> MFRRGLVHRRYPFNKRGPRERKSWKHHVLTDPPKPIQWRDPKVWTKDLTTMKSFDAPQWDLWQSRARSEDIDEALQPFMDMPQSLKDRRYDIPWWANPFGAWYLQNILSVELLKLPSRTNAEKVAIYRNQKHSLSSKKKGEAAQDDEILANIIKERWRTLEFGDRDAGYPCTFSDYIQFLNEWFKSLDEEGMQRLREHFDRRIRPLLAVMSPVDILWLEALTQNSPHNKEQLQRRIAFQTSLGTPEFFDMSKRLRYEINEDYKVRDELGPELFALWSKAPERWPPERLSKMYGLDFTLVRKILVWHHFKACYDACVEPDWTLPKRLFALEWIRDVRARKHGLFYGKMRFAEQKITFYSDRFLFRDLVNRREASYANVWEMDDPYRFLQTEQDYEDYWGDNYDVYRRMFPEMIGKSGEPVQQYGQMPVWTGPHRQHANKSQHNWMFAEIGVNVGHEALKKLELDPTNEKRRRFVIRQPDGTLRSAKMSEMRAWYWKEEWADFRFWAPNMEWGIENTPSQEQYQEHVPDTPDADFRKQRRIQSRPVKWFYESHYTRTGNFAGFQPLRFMQRRTEREVRWPDVINAAVQIQKRKPDAYIFKAIPEI;> MFHFTVGSLKNLNSWYAKGTMRGGVPRIYYAWMRPGSFTRRRFEKMRNPFVDLETGTSLYFRDTRDSAEAVAHAADSKGLKGMDNAIDLYNEYRIVPDLYPEGFQWKHKLNTEYNQWRSNTWLTPDLIPQEHRGRFLCNFQLNIVAYDMRVVKFSPKDHRQWIYCVLYVGSGKGIAGWGRAVAPSTQEAKKEAIREAFSNIIAVDLEQEGPMYPVRVNADGVRVLLYPAKRIVANFRVADILCAFGFQHAGCRINLKATNNPKSPTHTVEGVFEAVKALRSVSEIAASRGKVPHSLIYNIYPYLEEIRRRKGMMAMHPPGKDGLLMPDRVVDNRLPDHLKKGYYDDVYWKDFFAGSREHLNEPKMGLRGDEMRQRLESAQSRPISSSTGSGRRTLEDVLKRLGKTTKDLGSIPIVNPRLDIKLPTHIKRNYSLH;> MYAHVVSWTLFLHVFFFFLSLSRTLFFFFFFFVCLFFPFLCVYLEEEMLRRLVSSHGCSNGGGTNGGRCVRPVKEEPPVFSSLVLQRRFSFKYATKLQHDEMRQPFYIHEKRHGIFSNEKNIRKSRRGLPFITPLYTRHMNLWETDTDASKNRFFRGYVFGQRELHQLLGRPHGFEANNTDGSNDISAYEMTTDQRYKGIPRPAITNLHYEPEWNYTLYRAGTHGSQLSNPRSPLTAEVLGDELMKIRDIKSFDHCKAWFDRLQYLIKLHYDAVGDIGEFKSRHTQHVHEFFVAFHDALSSFDFGDSYLFEQFHAARPSELTDLFGIFLEMEANYVHEDYCPRCSLPYSTTRYCGEGDANTPFRKHRGRWAPHQRWGREWYAVVARRAEALWYRATEDPYFGTPQHTQRQAEALLRVYVQTKQRGKAIDFMNALRGSKEFLLGSICITPEMQESYDRLLDTTPHPHLLTNGFTLESNAAKYTGEVQKVPFSPLQFRIDMEMNKYRRQQKEEGAVRVPPAMWRIDTSAIVPYKVDPKTKRVINWREVKEGIEKSFLSTGLPKEAYTGSEWREMLHLKSIIAGRAAKAAELERRLHTDKVKLLEVSSKSKIASETNTSTGSSNSSSIIFPDKDGYHVFDTSVASLRPFGVSQSGAVFQSVTHTYPSPHAVLYNDPVHGKQFILDTTNESCHLFGGFEHGDRLLIRARKIDKNDNNPNSVLAVKGNEFEVIVVGVNKEGSDSEWQLCAMHVDPALQREYGLVFLGTDCVDIHERWASVRYAAAAPHVKGRVTLLEERRTAREESLGQIVGVRDGVLFVQWRLLRGGGSEMDRSVAEPIGTVEQVRNAYQITEQGVEELMHPPSWRTPFRNDFAEERLEELRQAPFKRENWVSLIQGRYTPKLKRFGYTQHTTMDDFETKEYKDRLLSKQFFHNPQAFEVIPDRRDRAVTFGGKWEYQRTHGLPTVDRNELENGWSEVEAVTDAEMHVIEQALRDISGRRPGNFIKSPTKKNTLQLNESWWEPLEFGWEQHNKEQKALVDPTEQRLIDSASLPFGGKIPPFGTTIGIGERIREIAEDYAKGFGLGPHGHSPSHDTCQYNTLNAEEDRVRELGYKDALVRLFDEKMADKDVHQWAVEQCADGEADVRQLLLSLHEWRERGRPPSLMLLQVLSKYLEQEIAAFNEGVPSSVPKLSLQTVDGTLSPSGNSGERSGTIWADVEPTAYALQYASQANHSSLDEPFILQLLKSAQLGGRNAQFTDPFYNAYLENSVVSEFQLGLAALAGKGVSPSLLAQKISQLHRGSVRLSGNVIPFVKSRELAHLLERMGLSSENIAVVTRGLANCPEQESVGDDFAVPVSVILSWGGPGSGSSTNAADRKGNATQSRNELQRKGSAALSSAIRQLGQKRSSSKNWQNEDKMMVHVIEELALRDDGLVMDIQYIVRENRRNPVLRHEFFAALLPVFAGKHEKVAQLYDEYCEGKYVPNITLAIEAFIAFLCNVTKHADVYPGSSYFDVDTTNGPNAGQYISLKLLDPLDGPFIFDNIKAEHIETVERFKQHGIQVGPVRAPATGFIAANSKSLSYFTRRPEEVVYVSTDADQGLRRSLERSAHYKTIAASPAMQFLLHTQNGAGLVATFNRFFYRTMPMLSFYQRILKHYSDNVQPLRQKAQNSVRGLARVLENERSAAMEEFRRNSERYWRNVLEGRSVEQAMGGSGGSGGGGGGTTPPVSSSPSQSSQEAMAADVARAIGSGRTGDQKGGAARQQQQQQQRTAGDDGGVRTTFASRKGGSRSMTDLLSKLNKPKGSNTSGTAKGPTKRGNPKSHTDGGRGAKP;> MIRRRLCFVSRPTKAASISVTLFSVQRQKGGLHTFIRDARSSSFTTPRQASHAEGEHTSSSLNSTDWATQMQRELFGETDPLGGQAHKDYYRDPARGYSPQYAPRNFAEGGAISYHHAQSPMEYAEATHRRSWLDHDVARMEAAFQEQRALLRGMESATERDELARRYAAEHHVADIVVENQSLLPSTQVHHSTSTSGSALRQQAVVDRFQIADQQSPLATSDGMGREELAHTYRMRSETVHNDWIEENLRIVHGLREKEKYDFTVLQRATRIPFQGYDMDRFLAQQKGTPYGAQSLPPNTASSTMEEAQRTLRDPTATVPSFEAISQKAFARNTVRDHPTTGEELTQEVVDTIRTSREASEWQREQERAQRFGLGRQGALVQDGGPDKRTLKKHVNDERIMDAMFFRSDAYRKTQTDEHWNPYMRQDTTHGVAHLLNNKFDIARREDRLSKGEQDLTERSVMHFGVPIQQTIDEFVFRHRNARGERPLDYFKPFPGFRDFRLNRMYRDVEGFSLMKQRPEFLEWELFTRYRAHHQQRRRIALLHGLEPVANETAQERDARREKLDEICERTPFDERELHTNDDEMQVSGETLRSWFGVYMLPSPTVVEAVVGASASVNLHLFPLADEMGTADTRENVLSSRYFNRLLLMEGFQNRISRAFMGNVSGKAPEPVVQYMQPPEVLRHFTAEERAMYEQYVKEQTSKQLGEWATAMRRRRWIPDRQQYGHVVAQGYGVSVVDLEHADTAAVLTVSAKAFERELAAAKGNTSHIIMVEGQAYKLRPDSERFVVPLSVRLESGEVLDMTDEAFGRYELELLPRNVNHALNYGIGDYAYNRGNYIETQDVIWEEQTASGEEGWSPATHADGLRAGLPVRARRHVGMNANGSRIVSSPQRAVIVAYDRQPFFNPEPRLVRVAFQSDGSVEEVPLANIMIWQRRYHGPERTVGDESRRFSPASLRRYIDVSDPFNEKKSKGEHFLDKYEAARTSEVAAGKYRTTKQITEIDQWTRFDVSRADNFRPLSISHRRDYIRLGYMHRYTPWEWIAVQEADQPLIAEQIRQDNIGTSYFFSLNRYWRYKARPHGYIRHFDNEVRDLFQFVDGVTPWKQAQKIRTYWEVRAHHPMPQFNRPEVAMHRNTVGLLPAHMWETDKKTGKVKAVKDSVRDYQTKTPLPKWVQL;> MMRARRVVVALSPLAQLCVHVQWRLYTPIWQPDPAVDHVAPLRESDENRTLWASSAPIANVSDAIAAWIRFGNDPVLHTALPVIHAGQNERTRTDGSSASLSLSSLPSPSSTSPFATVEDYMGTNMVFGSPEHVKDSAAVWASYFERRYLSQLRHSRRTAANHVGLVNAPDVFTDEADRPETKWSQDTRFRERAYMAEKFLKEKVANLQQLEQALKQAKPAEYIAFHDALQQQTLTLIPLPSPSVWHYGGARRTQWAERFLPLSHEAQQFFTTVLAEDLKRAGDAPEKVLQKVAAVFAEVGKILLQRHRRCLGGREWSALAPHEKDEFCMKEVERWKQQVEVGEFDPPLDGDDDPTSTEWQSEHDAIMQLMTATIDGLSFSALEFWTHTIRCEEMETEHIHTEKRVRAISAAARRAMYDTTSYEAVLQGIVDAVAKGQLDMKAAGFKPHMNDIWCQLNYAKFGASTVTQHTTTARRQLNYFHAGLLKEVAATAALYYATKPLSSSLDYASPYKFRRSLVGLFSTYGVEMVYAVQRPLLFSAANLAKAEDLIRGVVKNVARPFGERRRAKLKQLRANHRRLATPVQGVVVSAVVSDLLESGADVSEAKKAEKMQESVTFWPLGARRVVSYDWPTPHFDALKRRVAAAGSAVTAQSTKEIQEIKRNAFVEVSLWRRVTAEETKQRRDAVEEETRRVADVVRTIPPLAQVQQYATSLYQRIEDAAPFPAATDNNAKSEQEDDESSWEFVVMLDDRVVLNANQAAELYLPYTDASGVPIPQGECRVRVRGFDVDVNPTLNPAFCSEAFSTPFQVFDAIPQLVQQFFGTAKPSVAEVSDIPSSKFIQFCAFLREAGLDVPVQCEFEAGQVLNAEGDVFMEYFLNLLRSDRFHRSCAQAGLTEMQRVIESSCRAHWEVHHPGANEAEWAEARRRVLDRAMEKEREWWFPNEMLDVTNMSPGSNHGLRLPMYPATVRYGRELCTLLAAEGQFDNNSGLSATCAVNGTGAAESITFSTGDHISSTFSMEEALAVAKGALRNAHDRQNTLAAFRLGPLSKHSQVLLFCGINATEFGGKYARTYTYAFEKAKKELAETFVSGRVVPGVDEDELLRVSDKEGVDRFASSTHPEQRKTQFVPRVGPGGAPIEDPTADQKTQWGR;> MFLRTHVERHRSGKARAFVFRDPTLKMMRAGSGYQQLRRMGMPIQVSKGWRKVDHFHANNQYQHAWPLLSHDDLGNSDQSNNTRNIMYSMYLPKRNKGTAPWFRGADTYSVKYCEQGRYEYQRYLMINRFPSEYRKHFMNFLSNIRSSSGPATIPQEALHWLLRMIVDNFNPQHVHYIAAMKTLQNAGELDMARDVWKIMERQQTWPCTSTICAYLDVCVEAGEKTWAMEAWNRYCTELKFLQPGEVDPKPVSRVPFSLTREELLYLPKWKKHFDHDPNLDVVDLNRFNRTREVYLRMAQVMLAGGERDSFQHFYTKLEEAMLSTPTPVPEPPNPHLVRRPQWSPYEHCKSVHHSPWRVGNNGRAMALGPSLTTEDEMQSRFFSNDQFLVHMLKEILRIVLQEHRRRHPEACSRGEGEAFFDQVVDARETLNFCNELIERLFAVLGQKMHGLNTSSLLSVILELYRVMGKETGMALLRRANQFLERKAALEDGAKESLTAPNYLQVLMGFADESAYVYDSKRKGLCRYRSGFDPRTTMQQLAATVQEIAGNPHVTWAADMHLQVVCTMVGCGTMKANDYFVRNVLRQFCWDSRFLEALYMEYRRHDDVDMWAELTKRALVWTARYNVNASERLKRLIEDDYDTIQVHTRTFRELAVFQFRDVEEKRHSRDVVNELPNPWTDYVSHALPFPDRDAGYPDEYGDIGQWRAPGGPGSPVKGPGYYAPPMEGEHQRGYTAEWRDLKNPMRPPEFPTPWERKYKQYARGQHPSYDMVYAGPMPEIFPNRYDFRKPTRWDFHDIEKQGKYKTSGPY;> MSVTGVFSKGRGIGHAAVTSILRYIPRARVPWQPSRFGRENLSASDLAVLWSRGRYRDGPGNYNSGYHTEKTHVLEDNTVTMIPKHELEKYMPDISIGPKALVTPVSLMSARNGHRVTHDLLHSYDPHIGRLDKPAVVDHDNITVEDPNRVGLNAATLDCRGRIYRWLRRGPFFQEDHYFRRSLRLNRDGTVPTAAHEAPLMRKIVRLAQRGHLKAACEEYRRVTTVPPVEVYRALTACCIPGGLIADAVAIFEDGNSKLFYVARDGEVLHNVMRCAIKAKNRVRVMWVYNVMRGRYYENVIVRAEIDPIWRYRIALLALEYFLDHNCAEEAGTVYSYLVEEDLLQCDVHLRVGLHMREALSKGKSVGLSDEVLRATSLVTDVATVAPEVARELYQRHVEALRENEKSNDCDMNTKNDGATGCAWSAHGLLTALDFTQKDDALPWMQQNFGDVDVASVLRWARFYHSKDLMAKDRPRYLARAVAWIELLSKRSHMMEEAPLTYMRKSKPLSLNTNSNLRVAWQTPVARPDGPPRLLAREEGYTFHHNEHSRFVTETYRHPGETLQSRFLAMQPIHTEVSAKEDFQEIYAQQQEQRALPSGVVSPTARILHHSVTSEIHGGGGGQHHRSMSRAESSTGGAVKKEKLNLVSPHVAAEKRGGSGTGNIGGTAAGGGVTPEF;> MLRRAPCLLATNIPRSAWDPAHFNTNWSDSYSTEIAARRHWPAKKWSIGLEPRTPRDWLQFSYRNLAYAYNGALRACQSFPEMLVCYKEMKQRGVKVDVDTMNVLLTRAARYERIQVDDVFLLFDELTALGARPDIAAVETLHTVLDHSAAMPYEWREARRRQLVELYNCLAMEEIERLAPHRVDRLLKEQIKRYRDNLRALKASLSPSVYRRYLHTMHSASMLLEEVHNFLWELVESDHPAMEIPALQLRIPFVGSVMRRPETDTNEKLVKYTDFEDTDVCSVFLAAAERAVDADLHDTRAVSERRIFLSLLTMISYSGVLYTSDLMAQLMEMVKYSTHASSRDSDAQRLLRYAVRGSSAAQDDLYRSLWLKVEMVADSRVLGRYIGAREPWSPIRVCFDERGLFKSYPPLVHASAKKTSAIEADATSGSGSTTMEEEQRQQSERQRMSTEITSHTSKGGEEMVEGVRGAVVAETSEASGVKDVALQEASHGEQRTVEALDLRWGDIHRLIERTRALTSPPTERHPQQEKMEIFTGIAVYLRTIATGRRYCSGEEEAGGESPAESRERALFAVGYELDVWARLFELVQEVRHDMEKFITDNAAHHVEPEFECWEALLITLRCILDFCVVRTQEKGKEERAAVEELFEKTMKLRNELVEESRTRFGGRMRILWLQEA;> MLSQNVAKTTVPSYYMIRTNLPQRKPQNQWEGVYYFGGITKRQRHLILLQRKREREARMRAFSASCSNLLRLLEGDTQEQQQAKTQTIQLSSPHGPFDLAIRLAQHGLYQQASRIVDELHQQRALRMSHYGLLIDALSAPCLGQRILYGSAQCDPALTYKLLGDENGEERAQEAHRWFDMAFALLTTECRMSGSEHRLPQATAAATHLVNALMRALLTCGYTHVSAVPDAVYDRMGLMGISPTISTYELVMLALSLQGNMKEAESVFSFLRRHHNEHVTIGSFNALLLGHRECRQFDRCDAIWQELVDRRWPRASTLTAELYLRSIVDHSYTPTSGPLQRFGNINVVEKKKIPLVLAQMDDLGIPRAHLSRPLMDEVEDALRKFHIYKSRYYEWGRAVKQFNFIEFRRRNGWMYDLHLMKNTTKQVGPLRDFNQPDATQAPVATVEIPAFFNERPAWEQPPLEETLYVTESRERYDDVRSGDIYEDRTRSLHDRSPTWMNEVPETRYDHLYGVNHPDIAKIGIRRHLNAEYVNRKEVVERDAALMKKNLSTGRRLRRKVESSRTHRNAGSMSGAAPASASR;> MRSIRGVCCFSSLYTTQFRVHATYDVAPLSHKELFSIYQNWDKTRDELDLLEEVEERISKWKLNKWEMRIPPLLTAREKELMRQQQELLKSIFFDWGKCRDALNKDLELISSITGLPKGTVREKNRAWLQEEAAKLRWVGEVSKATRLRDAFLRLEVYGSRDHRLLERLCCIYGLGLQGSFESAFSNYIVEDPITKKIYVDEKNSFRDLLAYIIHTYPQIDIIYDFLGFNFIGGYRSSLRRYLECMVSRSTEGEKIPGRLVFGRGKPAEILFDFGNSNESLVSGECTQGFPDFVFVKGSDMTLIIIASENSWLRNRQLPHRKQMEGIARRASFVLGIPFSEVRVRNLLLPPTYLDKDSIVRINEAVLGLSKEEQRNLAPWLEMYQKELDSKDVDFCSLMKSTNEEEWLTL;> MLRRTSWRAVGYTPVNPDTSPMLAYSQYHWHYNLPQGMERPHGVNRTMTAPYQSAHSLVNKYRGVWIELDMHPAFRVALEPQLRKLPQGRTIPKTSVDEVISDYINTAHLIQDEMTRDLWLAKVLQHCAFQRSNEGMALWEKYCHSRFIADGATATPPLPLVKAILFYCSKIDYQGWSSIFQKCLKNDWNYTPLFDTAQWNFLLKSVGRMGDEKGVRLILEEMLDVQADLDRVEARSIVIALNAVTDNDIYEYIKKYLFNFGERKVKFLRIIYSDLRGHGAGKLRIPLKENDKMFYHVCWHSSIRAPRQFSPRQLYFDYTPSTLGASVHNPNAKIDDIVKDKIEKWKTEGLLPEDYVHEDRVYDRGTAFKNVARQEKWKKMPRIVKSKKMGYTGDP;> MSFRYTNGLVGALKHRMMLESSHRELVRRRFTGHCRGVEVVCSGYGTVLAVRLVDKTVWEPFYRKGHPSPSGADMDSAPPSSHAEGTPVGGQSAAPLDFERIAESIKAALWDATRKIRSAKEAALNRSLSHNQQLRAQAHLEHWYDEDANTLQPLAFEALKHEAATPWMQFVQFGKYKHAAAVMHSESGGKTSEAFTGETKRAGADNEEGPCVTALDEKDVDPTSIPIGSVHPLFLPALIQFESRVDNSLNDDAIRQEQRREMSRDEQLFWERVELIRKGQVATIKGGHKRDYADEAAVASDNAVDKVQLRFTQ;> MMRCCCVLQDKSMFAAKRRVIVPIHPTPNYPAHFIKASFTTDPLKEKQKARFSSGGEAMREVQMIPKNLEGERSRRELMSRGDTEFEALVEFIQGASYDQLISGRRFKKVYDKLSENDDTFVWLCHTAMSVLNPGDVRSRLVYNHLRTLAEAVANGEMTLRTAFRFYESAVRSPAYREIAKRQMEGGAATRLAGISAAADVMRRMGLTRRPMASYFELYQRIVERSEAMTPWGFPPLFQFEERLSLEPRLKFFSRASQQALERRRRGHIMSAYTTLQGRRIFWIPPTWNRAGRFLGPHVTLYPGMTPD;> MEVYRRITERVRGALWAHHGRLMSERQFHRILAYVYNNKYEHQIRFDRMEVVGRAWEGRVEVVTTPAGYLKRVRVNPCLEELSSYRQQQLILAAYADACAQGRRLMEKAEINIYKQFLKDLKPIVMGIRDNPEFYTVPEDSVETVGGTLHMGQGPTPTTYRTIPAAKAHIPVDEIRARQEWEKKWLNSPQGQSWALTLRGKRYFALHGPQYRPRGAPGAKKVTMPLDLPAPYTSMDERRLLKKNWMAYLDNKHVAEVMWTRAKIADREKLQRRLQETGQAWHRPINKEAVSRW;> MLRSTRPWRFRMKGGEMFVEYKIMSRDHRRSIRVEDAIVDPSVARTVVPLSWLEQLRSPSLRLHTGYHMEEAVYVPPAYAAVDEKEGRRLSEKSTMTPNAILAGPVVLSITGQSVPVVLNPYFVPDDTWGIRRNRDEWDLRLGMDAIEQCTLFSELRPGGLLYNKLPSSQNVTRHEPVRATLQRYGMKCGLAESPLVPRPWTRMRYMFIDELQRGPKLTEFVGHNPRNGTQWRFSQHSKYFRIGVWRETIRRNDMNEGLHGHSSWQKSPQQAVPEVRLMAPYP;> MRRFCFPVATFAQAALRHRGIRWNTTMADNESHTGAKSSASSSTPSEANEISAMERASEARREIHDLWMSTEKMLDLENRVRSVASLIEKYKLDPSTPRENDVSRGLGDAFDRLLLLCVPLGKDSSKGTDDLERLMNLAGRNGREISVRTIQHLFARTDSFSEALAVFYAMRRCHVAMNMEAYYAMLYSLQRLEEEGWAQRFREECEEKGGVSEQAMDFVVKGINNALLPENKPWLGRVMFGDRDAPAQRREARDYDELSAMWTERYRDGSAFPTSP;> MLHGSLPSLASLRYRRPYWMLFLKDVDNWKIYTVIQQPDHQRTEMLYQAWLGGLDRPYTRPKCMANQPLWLSKKRHILRKDRLDGPETPLEKYVLEWHKRFHSFQGTERPTVDDLHTALDLVERPLDLSYAFQLLNQCRNVNNIRFAKDTFLVFLEACLRVDRKDCALYATENAEALGFWHIEEDYRRYLRGEQSWYRLSPLDNMYYPLEENVKLNAGRSPPSSAAVAEGDAEGTAETTGFEAAAGAAAWSDDEGSMKAGSSRESMTVDDEIARLEAELAALEEEGTDGDNDVKGPKGH;> MLRRTFAVVQKGERGLYFPINHRIVDRRIASGVTVEEADVQSRYRRELRTSFATGETRQTIPPAWSACERPTHFLSLRLPVRNVLRTRVNEMHNQILFSHQQHAPLLVPLEKLHITLGVMAISEREETERLASIYDCVSEVFSVIHPLQLRFRGLGTFGFGRVLFIRVVPEADFGILETAVSKIRRRVGGELKVDMKGNPHDSYVPHVTIAKIRSKQQTQFGSKIPISMWVEYQHHDFGDVTFSQVDICSMRGSKDGYYHTEGSVHLL;> MFGRSALCLAKRFRYNTKYPSLVSYNKLPWEILNHETPEFHMHVAPHYEQIMTLAASTHVPHIVGKKHLEMPPEHRLRLLPGMFYMLDGDSIPEGFTANRVLDPTALQYYGRLESLVAPVQAVRMLISDDLRIVCNSVTLQGPLQLPVASYASLASLEVVTNKASASFTLFHFVRPNRPPSELQLEKYYIHAPRAMALAEFNSTSNTSWEPKLQAPKRSKRVTPLPAYRPPQSYLMGLAERLAVVPGSSFGRRSLMWGHWF;> MMDRTRLFLAAEFKQKSRWSSVWPNMHYGAMYLSYSIGRKLPMKGVNWVTRESNRLTNFSNRYQAVINDIDVKKTEEELGITLQDIRWNDHRRIYWKCSFCGSSYRKSVSVRTKFHAGCNFCKGRYPSEVLREQHQSLSLAASAPELIKQLKETDKKDNLGSLALTSKFRAEWKCQSCGGSYRASVRSRTGMVENGQCPLHPNIVDWSAYCPSCSWRPNMEAIAEEVQRTGQFLGLEAESRKIASAPPARIPRRKKLVS;> MLVSCIRRQADRRTRHHMMLDGQINPREWMNWHPKEYQPWYFDRHKFLYERQQYAHFHHLLCHQVFLKDMLHLVQHPEPYTHIVDCRTSPLKMHRWVPHSWWLPRDEVEYALQLTPDEFADMYGFHKPRKSDDVILVSHNGLYSEQAGWEWKKQFYQHVYNYRGGTNELFGEQYNDVALKDSLPPWKGPFPQSGIFVDKWSKRKVLTRTGPFDRQYEMQDFALPDLELERPRHPEEGPRQNMPYGLQ;> MFRISPSLAWRRTAAFYLRAGKLGQYEREAFEARRRLEESKNYPGPIRSATPGDTRFYAGSLESILQDNDRHYWRAVIDDPQVQYVIPLRIRFKLFTWVTTGWEQRLHIVQTMAPRDITIARLIELVTIENQSPYLCSSTFTLAVDGKELDPDKSLSDYGITEHSRIDAIEKLDHLLHKDSERPLDWTVDEMTTECLKRSPYKEMGMQPQPNLAPRYEARPKGYFGRNNYSGMKQES;> MQRAGCGIVRPGRGCHTTPLYCSLATISTGVFDHLPFQHRRQHAFNTLPLHDANHFGGRTAYLREIGPVNIKKSGRRFKKDLRTVQFNVDIWCAQQTLRKRWKQRDWEVIEVPFRLAPAEQQRVIPEMYTDVPPMTDPERHDFSNIRNKVYDREELQGVLFGASGPLPYPPLQRIDRQAMTLDKFL;> MRRTIAALTATPERFSILGTTHPKPKRTGFGRNNKMRSKPSDNVAWYDKGPVEWLPRPVRLTYDHLDQLRDWMMRETLDGKTEEFNRIRDMHREWSQHPLMPVLGDVEPKFPLNLFKQNHRAKRRFLVRWHKANTPANWLWMPRGPTVVTPLHHTNPSQYPESWRQMVRKKK;> MYCYYLHTSPASNENDVCHSASAKSNFIFPSFSSLVGFIVFFLWKRQMPLFHRLFVSGADLRGCHTALSSTFTQRRYWAKPKKRPKVGQGFHEKAQKWRDEFLLDRHRILADSLRAYVEFSASKRTEPWDTRFRPFDRVEKDGVYVLMRHLMEDKFQLCNYHHRPVKRLFCNVGLLGPQVTTKARWKPYRYATNPANTSKAERIFQKDKTLYTHGHND;> MFGTTRVWRNTFLTKSVATPPISVIRTGPKWWADPERMVRQKLMYFTLGVDQLPLRRTAVIQKDLHRFHMCKPPPRIGDTTGYKRSRAAQLTTWYRRIQYQEYHLQHLFTRHVWGLVRAYPGNTTKIQGKADDGYVGYDSVPYHRYNRTPLPFPAREIYGRRE;> MVFYAFVLVMKPRQRRFTSQALREIAVAIYNNGGLIRKLSNEGVMRPYSRFRDADNTPLTYARYVTLQVDMGEEQMRKVEKIMKEHQDVFITLNLNNLERPVGIRRGRKDLQSAYFPLDTFTRLEEEINWPPQTSADIYKQLEMNWKEFSRTRWSNFLRN;> MITELRTKGATRTPAIRYSYPAPPPSKNAAPQQPRGTPRPRTAKTNVRKPKRSDARRRARAGSGFGVVSPVRARRRRVVGPPFADFFGALFPATRGIAFLSDLPTHIFSSFLLSFLAGRGVAMLRMCRRLAMKYADLELTTRGEFPHGMKEPGFVKKLDQNIPWYFSTYRSMYHWPITGDNWSDLNEAEKHHDLHMFYTLAWWKLGEGIFDANDEDN;> MRGCGVLCAGHKRAAVIATTTCSLGPPTLSPSLTLRPVACAATPVTIPIFPPPMRGSFIDRNPVWASFNEKHTAKSFRHRIVSSADVSLRPPQFYLSNEKVSAGEAAVVQKRAEATDSYGEQLDEISARWAAKFYGRVTFGPRNYPYPSSRWLARRFKMKKHRIIKRFRFRRYKLAAVANLPFAKMIRVGLLPELKSSKTKKGDDVEADLSGRLVSAVRSSGGKKKGNRGRPKSKYQI;> MKKMVFCKMCRPLLVFCATSCWRRSARLPLPFFFSPLNLQVAPFTSWNLQARYFSTTAGGGREGTNSSEDDYVFDPTLSVQKDAAIHVAKKSLDAIVRDLLPENAPDAATQKVRAYLQQHPMDTLITQPTVHITHVEDPESGRETKMSLSPCDLSEALEQAQEREMNLVQMGTRGDVAYCRIRREIPRILGLVGPELEALREEEKQEGSSHRGGSDQAGGKIRELVDHSFRDVVDAHFVGWKSKKIVEDIKKRHPVKITIKEFQSPEAAIGKIREMCQAMQRYAEEKLIYHHFTSIVANDREVSVSFVPSLPSEKGNSWKHIKYPGEKEWAHANKRMEEACRKSGRYGTYVKNNMLKPRSLGQTFFRVDKYGRKID;> MTKKGATKILFIYKLSKLNVYNNESYKIKLLFNHLYCIDNYNSIYFNLNGILIWLNVLHINIILIKYAFLILLNNLEYLIIFKYNIISIK;> MWFLYGCCLRFVLFVLCYYMSPRLPSSGNRRVLYAVFYLYIFVWCVRCFFCGIFILSFALFIIEGGGFIDLPGIKYYTRICY;> MLRRTIVPLAKVYGAAPPNGTGQMQPARHRLLHGKRERQGSLFAIANDVKYDEKRLRQQLNAMLEEERLPPRTRLERNKANGGEALPQRRLVDLPGVERRRDLPADPITRLFFQHKGDHALYYGTYDNPSLQDEDRIQIEKREPRYWTYNVFTPVYDFCHRIREATEQRKRFVIVPSTVETRGCARVMLGHGLVAGFRDFHNDRAFAVELKYFQGDSTINVIEPCAYDGKTEFEWSPKMMRRLMNTHGIHNRLVVYICRTADNRVIDHIQAVKENVGGRGLIMVH;> MYQLLSPRTARHARLFRLANNLASSPSGTAGVPKTDGERLLWVNSHVKRNKDIEMSIEEESLRERQLPLKLGENAFTSSAQATHGSLFHFREYPMYPGEYVPAGHNTLSSLRHELRLELTAQSLKEAWMRISGGIYFQSADDYYASVDGLDAEQLGEVLAALFPYLSTYEAQALVQCTLDSISKPMNTASRQLSRTITAEAVGLDNAPGHYTNFLDWMGRLTETRGFKTEHALFQFSRRKFNRDDVRVMFENYKLMSRATLIADSADSYSHFYTVLKDFARKVAGEDSRHQIGVRIDEPEVDAETGIAVGRGCADGEKYQFTALLRENRDHNGAITIMGKPMALVLDNKAWLMEMLLMPFDEANLDYRDFDVHIVLEGHAMPSIANEIAAFALRMSIANALVKLLPLTRIPLKKSGLLSVDRRRERGQFPGYLDGKKVKRKFAKR;> MRRGIVNHYYWSRYRMPTQMPKFDGPAPIAAPQNMNSTKTNEFIDPIDDKFPLSIRGPLVRPDVPEDQYVDSWYVCTSMTHHLGDYRPWSASAPPNAYRFRPYNEFDAKGREYVEYMRQFARYDPRKSQGKGQKGFPFRDAYLTKMNEANRTTPPPTLETIMDRAVREKHQHARVLSPMQVQRDVGRSETPLPCAGNIPVDRSQFPFCWKTEDWYEYEVAKVRNKRFVFENTEEDGIHGSEVTYKIVLEGFWDHHVMKLAEDVCMFLRDVGRQVTEEKLVAVRRVMEGLTGGAFDPELIDFFNAARAGPFGRPDEYDAEEVANFVRADLKRLEEQCLNVINRCNVPVPGATNIYDPQVSWPYVEKLEPWVRMAEFWTSSSDTSFTELEMSTAHYEFRKYFRVIICKLPFQSTEFEKRMYDIRHWLHRQTTCEFHTIYRKNVIHDGSVFPTEHDPATPTTHDHHRMFSFALDWQSAPVNRLSVARVLEGDDWERVAQRLGCSVDDLKEANPAIEELEAGAVLNVPGGASRRLTSFGAAPRVLPLQNPNNGKRIRTWEDAATVLDCTVEELQQANGHAALTYKQTGENGEGEFGPSVTELNVPLSCWVSTAETEFSPVELVFAGDTFATIAQRLRCSEEALKKANDGQSDLSHARFVRVPAEAKAPRRLLEPQLRSQAATDVLMTRTIAEEAAYGIKNIPDLPSNASKFPHEYHTPTSRFPTTPKEKESESDWMAYTARYLDKQFTHPTEPTPIYNVNKLWPMQQVPGKIDQTPFEEDQTWLLNPIPVQQLEQHHPEKDLQDLPFVNHEQFPRSLEWTAP;> MRQSLVLLRRGKPRPRAGMFPDKYRRVPALLKPQQGGQQFFNQFLIRFTNDRLMRRDVEDGEDKKESKIAAQLPQMDWEHMSARSSSDAIREEMHRLVEGDAVQHQRVFNERIWYEEEERRRLQTGADAAAPTEDAGGAKEHDIPPRVLGNDYFQSRFGYSLVKQSEMPQGVTDYNQLDMWGEMPKYTRDMVFLYLISRRRNTYAVAYTYEGKRILSTYTAGNRGLKGGDRGFRSDGSTDNGHQVTSMYLNDLLPKVRELRANEGRPIGRGEKIELVVRVMGFYNGRQGAVRAVQDRANEFHVRYFEDITPFPLNGPKMPRGVFK;> MLRITSACRGGYMMYHRKSMGTMKYSKWKGAHGGVSHFYGRTPMVEEVKRNEPITLIDRRIMHYVHRSRLRHFQLFRSYQQKSNATECKLREGEMLRRRWHRKLQKSFIAFMQFKTMKVLEDQAKLVNTYGQAAVNAALGDSWDAVSDKEKDRKYVTIRRQVKALPVVSVVPKHVATMKQIHNDRFNYRWRVN;> MLRLSVGFLMRHIGQDVPKRHTHFVLESRLMYEKSFRDSWLHSVCRAVSQIDEPLSKTISGTRQKMLQRKVTCFQYNQYGLFKVPYYRLANVDRYHAVQGVPGTREWVPYANVSYWTMNKMVRSGNLLVHRVHYTGWGTDPHLKKGGWEHRWNKVMQRNALQYSRI;> MFGRTAFLLRKYRQKSKAPDLKTSFSKTRNFKKAEKIAIETVDGEVVKGRGKLRRRSHSALKKAIGEMEHPSIWLWYPWRMNPEPPTPGMPQRRALKNLHGAVFTDLTPVQKKRQEQMLYGINIPETRQMKFEQEHPLLASALRQLDGQPKGFPFWYKKYPTRRHAYGNRFSIPDEMLEGYGEEMKKALSKEMMSIQEKQFAQEAMYMERYAEHDFDTTSPAVLAVKRALKCRVLRNHLLTNPHNNIIKAVLANTEKKLSHALRKLRKVDFKKYWEIIRDHDVQDVLQPSNLVTYRQGAYWKYDWNAGLAISTNLADVLDPRGLNGCVETGRSRSEVARDLGLSYTRPLQENEKKQLSHQALYYERLAKFKMEQPEAARALERERFVRKFSGMFAKMDIKSGAPDFPSTYRKLLGTKVVRWASKRHGPA;> MLHFTSLFRARAIIKRRTPQLWGAPGAPIIRMRGHHVVWKFQSYDLFVEHTHKRRNSDARLLHYLGKHCPHPQKSLWSPDTPVAQDRHLFMLTTV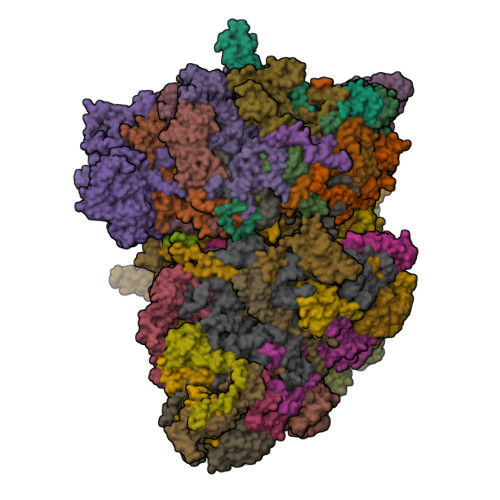DVDAFKYWFGVKRCRLSMRPWALLAKAGLLPPSLRQNSKIMPKPIFDKEQLMRYYLANRKEEATIEREDYLNYKNSLVKSEEERAAERPVAPYL;> MLRRSLVTFPWWNFQTEHRQRCVMMYGGSRAKNTHNANHRVFIKKYKRNAFPNRTRHHWAVSMTGVLGQRPRRMPWPYDLTSLIFNQPRQGSDKIGYVVGTSMLKTAVVAANHMVYYPKFNQRVSRTSRFFAHDEDLACVEGDLVHIKQCRKISKYKHYYVFSILEPNIEGRERLKLGLKAVPPPLFGYPVSRRIVKLNLTNAEGTKEKLAAVIQEHVQDAYRFAGPTPDQPRNRLTDSVTFDDANNMIAPNAPATPESLEGGESPSLLGDKEEYTEVEQDTRNKKGDEYWMNLQPKEKYDFKGFKKSP;> MRRRTVISFGYVRVAASAVGVIGMGANHRHHYQQQQRPITTRGQFNPVHDFTYAMERGVRARDEKTFEKLITNPGPLRIAYSPDYLDWLYRCYKAKGKYMDARAAAEKKFNGNIISGGAVTTSSGEMIHPLPGAPPPGMFLRPPNSFRRLSGEMKRKHAQETLDEVSKAQGMLDLFERQPQFPAIHIDRCTRFHLVELFKEMVLERSLEAVAIWDKALLYRAILSERKASYPASFRYIFKAVEDTVFAHSSVNCPSLEAYYYFLYLVKKYYIDNAVEAHVVLRCHREPNATDLLFSNPPPKDEVDVRNAIEALQSAEATSHAASSATSGTAKHDDPAATDEKHTRGDNDQKDSANANAKHPCQFAPPSSYPPIEALWRCEENVPLLEILLFGEFNLIVSENPFVKFPTAHAFLTRPYSTESSKGPIDGASLANVIAEKRGHLLPSFPMNVASAIDGRAQELRRLQQKHHRDDTVSFQTLLRSTHVDDNPSTFSSYSDWSYFNPRAVRAEERDRLTRKGIDALKEYDSATEDIYRRSFEDAQASNFQRVTEAWNTFPPYLPTLPHFVSIIKKDSHISFLLHVGLPERCSSAEAAAKHKEFERRIYQLARALYHTALEFHKETVRRVNRQKVNVAASLLDNFFEQEWVAMLRESESLENSLEQGAWPDKKTDMARRLGRYIPFARRSLDENGFPTDARADDYARWMEAPARMKGAA;> MNRMGGSVYANAMAQFAICRQPWNEYINLLTKQDSTPYHVEPQEKPAYRGRKRGREGWLFGQQVQLHYHRFPDEQLLTNLTRWRTGETVGDIALQQFRNAQPFDIEDKDPQGMQRPSPEVYMKLNYKNPATISRFLTRTGHMYPADILPLNPEAVAKLRVAKAQAVRIGLYPRFGNPFWFRSQKFRPKAYQENYDPTTYSTKHTMEHFAYNWVQTDRIRRYFKELEELQKNASNGARGGSATTAEQKQQNQFYAPENQPISMHRNNISYMAEVERSMKNPTVPGLMSTKGMKKKFHNLYSSTSTKRMGFSNPTLGIKKV;> MLRRCCPATLHVAPSTAMVAGVFVNNQKRFLKMAKSAFGFYLARRGQRKFPFLRRPHIKNTHAMNLSAPYFWSFMTAKSQTYFLPEENYITGDWTGKFFVSKLQVYTLQHATSGSTVRVKSFPSVFELSSPSRWNIGKELNTLTKPRMDLIDEQMLTKKQRLDYVKAGLLPK;> MRSTALRLYKMPKNMGVAPRFDVWNESYEPWQHMKRMGRLVGTGFYIPPEWYNHFRMFPPINHNFQQEKTLNPRNESEPTQDDTGSLSQERAALRDELARKSRLLASEGMRYYNIFWVRKPLDRMEKEYYELKRKGIAHSEAIKKVLEGFYKELAVKKRVAAVQAEEAKLSGRFITMREATVVLNVLAQLHREQLTPHQVTLLAREQHQATEKASGLTATVSRVSAPAAGIDADSTASKESGSDEALSADSLANMLEDDHASGAGTQYQVEVKHSARDSVRQLHEKSTDDTGSPDWYTGASPVYNGAA;> MMRCSRGCRRQLRPYYNLPSKSDHGRKMTGFLTPYRHWMWKQNELWRNVHEAQFEHLRKVYKRQWLESFRVNADEYIYKYNITKAAQLAQWEYEMQAQEKKRLEAKQMTEGRQALKKKHLDLLREFHERQFFFWYERASERLQSMNLIQYIPQSRVQEHIERELDKYVAGKSEAYPLNFVGQMPLVEDREGNIVEVPEGLLTNHVSEHPESTVKPHQPHESTSVSVEEQLLRTMASAREESLEEWIDDSRALSETIDDISREEEQRDEDTRVARSMEETDNEREISRRMYIDRGKTGSKAIFRRPTLSETDGGSASIPVGGVAASPADTSAPMRRRKKGKLDKAHALQEQQDAMIARMSAKSLKDGESSISIVKRGEIATSRGRIRDKAAIPTQEVLMQKPELAAGSVPNARISFKDKVDQLYHRGKYKQKKEDDNNPNEDL;> MRSRLVGKSLASLYVRPPVTCYTDACEAPVAMWNGAIPLKEVRVMQKGVPVRYVTKLYSHPLEASPTRLSFNDINSMYCVGNDELMQFFPEGLGGKVMQLMPPGHPRGFLYRKEAHLLNLFIDKIQHWQAKRNVLSSLTNNRPGFIIDGPKGCGKSALMCQVVHYARSRNLLTLYVPNAKEWTHGEWCWPSTILPGFFDAPDAARFFLRYFAKANRSTLLSWRLKCTPNDLPVEQGERQPQNLYELCEWGHQVVAPASIDRQSVCVKFLMDELSAEKKLPIVIVVDGWNLFSHDTHFRYPHPDFLRTLASLNDDSTDIDLYPQELPRIPASRLGFVRGLNKMILSKDEPNKFFFTCTTRDFKPFDGISGFPDVETDRFTNSLDEYAPYDAEKDSLFHPIQLGNFDEYEFRAFTRFLVNSGELAGLGWGPLWHFSSDFERKLYKIGFLSNRNPQGVIDHYHQELVWRYEYQRTRQKQYLLHRNMELVVSKRKNRHAEPKGG;> MALRGVPIRLGVHRVGYTHPSTLPVPCAQRWDLRLARARIFQEYIEEKAPGAWQLEDERSMSPEFKTFTGYPMREMRPGYGQNLPDFIMKKRLPNNTHYELFARRDIPNEDNAMYGKYLYDMTVHGTSLPSTYRMHKDINKAQRNDRKLSGNRFRVLCSSGAKKPPSGWEPIPDATEEEE;> MLRRAVVALRRDALNGGSSMTLGSKGMKLSPDPHRRRMPWTAAKEYVPGVVLNAKEKMVLDGVKLVDVECVDRASQVDPLEALRATVATYEYNTSTGKNIFQLASQVEFDGRGQRFYRKEWQEGTYDKYVTLSAIDFNRDGNKGTAYGYVTFHGETTTRPVQIDFADVPGWHMEFRVERAVPFNAIVPPPPSIGTDVPVDPRSYRLRAYPFYDAPNPPEFVERLLKDRGVIPDSPVETTELPNESEGSDDTTRRKN;> MLRARRPLPLLPGSRAWLLRFYSSTRELCQLQSRERLILGTHGAGVVQHASVSQPLSVNFQSSVTVAAPAADLFRTKVHEGTGTSGKDPYLRTLPNQESREPESSVSQAHITVAPTVDECSTLDRRWESMQYWFNDQHPRLVIYLRQLQVQDVPPISPAAESLLSKFEEVAIPKLALDDTDRQRLTKLWGNLTEEAKALRLHYVFDRFAFESKLSQLCKEALEQMHAMSLSGTEGSLAVEALRRLTILKRNDYIQRHLIDVTSNGAYLGFGDAVWRVFFSAVEAHKAVLFGKGTPDTIRFAWESILQEDVVRVPDVTAPVALFLTLVCIHEGNRLASVEWRESSSSLDEGICSSDNTQQRPLLALLNPVVKRRFVTKMVEFLLRSHSSNEFSKLLRKHGLHDLSRDVALCEAMNGSQGILEDDVAELVSRFESTGEVKTLLSSLIGGKDAAVRETVAKIMGIPLATTVDWDAMMQSVDWTNNWRRLATKLLCDQTLLVSIHKLVKNAIGAKGISRHLFSEEYADQLQSIIAIREERELNRKLKIDRIVRELSSYQRVDQSCEMLRQLGVDMKELDQAALSIRQDGLVKRPSVDENVISRALEAVGNRHPNWVRAGVIAPGAIKDSIGALKAMLFIFIRLSYVPQTGLAAMAQRFRRRIGPIGVESFQFNIPTEVGFVEHYNNLEYKRYDWQGWYQRMVDVHNRNISLRCRVSDLKRLDPNGVPFVDMQTERRLRILAEGRVGMGVLMLDSDKYEDQKDNMTFGSIKLSELLSDARKAQLGEEYWPSVEMKVRKPSGQSKAHYSLIDYDRIEKKSRELYEKYRDAKKKSLFVTPMDLWLEVKGMQVRKASDGADADGYTVDILQDALSSEDNEKH;> MKSSDIFHAYRYTPVFLKARQHDSGVNQYGLKPVNAYDFINPTNLVNFGRGTSFDNLGVRRAGRGEIDSSPSLGGSPVFTQAKLVGLSGEEQLTMCQSETMALRVCMARGGQDTCERESRALDACLSRVGHLRRAMSEACGEFNDWFIQNVSDNHTKPFQHRPHDWRHFYAQEKLVRERQQNGHAYGRRPKQFSFGARYVKTEGYGKRPRLPYNK;> MRSTCRFFDQTCGPHKSYKYTYMPDPRKLAPIETTTRSEILPLVIRPPTSYVPNHETFLEKVDIHRLKPTSDFKAAFKDWNDLMSCDKRQLRVRGIPRMTRIAIRNAVHAFQNGNPPEYFDTKEEWLYYKQFKTIDFSYRVIPELPEKYRPHQNGIDQAPLPDYREINKMPEWARKEEERLKEKKI;> MAVEGKKFDGREAKKGLFFSPHAWGWITHGMFLLLLLPMPLFFCSLWTHLRECCCCPSGPLRLSSGHVERHAKGIVQQMRRTLRHGYHAYVPKGALLKTDMLASSPQLVTAVFRETEAAAERADRANDYAGFFSRPRLNYPVASGIPAFISRRQFDVQYNIFHHDAVATLNRHTLGTSLEGHSLETVIRRASFDATQAAVHTAAAEHFNYCFFYKSLRPWGTAVPKQLREAFQLQYGRDGSVDVVEEVKRLFTVVVLSHQERCGWVYLVWTGKQFDVVEFPHGACPIGSDLIPLLAINVHEGAYSLDYGPSGLEQYAQNYFRACNWFLAERYYLQATGRGSSCDA;> MLGITSALLCVTAGRAALVASELQKLVPVLLPLLDPPIAKGVNVSAAQLIVASGHTSRRNDVHLPDCPVMAHALPLTALAEHSAFLRHPCRACLKRRVHFLSSEHFCMHLEEKCSQGGGGMPAEWESIAAGQFGLFTHFTDEFVMYATSRREPGWTWLVYDKERPEGHRLVVVNFPANRVPLVLGLWPLAVINMTESRLLSAIGARTKTSAAESSPAPWSRAARNPLVAEASTATVAAMAAAVTDTVDGLDGSLSSIRAQVAQEAVLKMNWGFVLQQWKQAESYYESAERERKVQAQRTKMEREAALAEMSKLRDSGATILTSDTVEITVAGSDAVPEKASRDLKASTQTTKEPRKEEEETAGVGTANQDPHCTQLEDGTWQYAYKNGDLTLLRPDGTRVFKKSDLTTTVFADGSTLYEYPNKTSILDRVDGVRVTTFADGTTKEGRYK;> MLRRRVLPESHRHASWPLIYETSQHGIKTLDVREYRPLATPIEFRFYQRYANHPNRQSGIQFLTHYNTHQRFRVNKDYIDYMHWGKEQGQARLPHRHQRVAFDFDDQLHPTRTLDNEGDSYAWCAEQDPTLGPHPDLDASFDPNRRVFSHPEHWNKMFSKRRPGEGRIDLRVLPSQSLLGPLMEQSDTQGAAYFRYDNRGHSNGRVPGLNTPFFGEFDRKMMQAMSRPLNADRTITGNDGRFSKTIMINEPKTHQALSGKTASELSVEIDKATNAVHSKLTVLEAAQSGLTNYYCGGLNFEMLGFDLHMAEMLREKARAILNGVASVSSTSVMVTTTSVPTKAQEREVGQLLRDALRYEDRVDDAIRQHASLIWRVYTAPRPLMALTNGKCRGTGCGVSLYSKYCALKDASEFIFDGPNLGITPYGGLTRLLARPETSLKYPGLAEFIMLTGTSLFAGDALRLGWTDLFTTLPDMSYHIKDWFDTTEHMHNDAVAWQLGHLLETCFKMKEAHSSAMERVAITPVRARWIEDSFADQPSVNHIINTLSEIERLPITAKQNTCDQTRCTPYTLTSVEAGISKLENHRLRYTHSPWDITPPEDEVSLQHASEIFNAYVLERRGTFNVVVHRDTEKLAAWNRQRQEEYHAYRSLRAAPHPRHVYARLEGCEGKLVSFDFVFSLQGKQKDQRSGNKEGEELQQTACLDALKRQVLTSFGMPDGRDIELGWYLPTLDTCPIHNDVEIMQLLHADPGIEDPKAQLKYPPIYFIVKRNCLYFSEWAYAVKHQLLLQSPFALRAAYEMLLEVRGDGSAERVMPLAESLATEFKYISRLLRRPDFYRVGVHTDKSAEAWEEIREERQRNLHKTHQPTRPLPDFEDVFERNVEIDGHRFLLRPRWSPRTLQEVLDADVMRLHTSLAYQDEGIAPLHVPTQCAKANRISDMVEDAGGLEVVPGLGELDAKGTPVVPPLQSNAHVPQNVSFYEMARHPWEDAASSWRRDGFTEGSLANYEAQYRAAERAVYDEEGRGGHNYWPSREASEGVTSEEKDAALLRERLFKPLEEALSGVEPWARNLRRSASDGKLGYKTEIATPEEKIYDDEYYRWFIQPGHHPNPTGLTNVHKGSSTLQGSDAAEFERIWRHVVSGVDGGNASDEAETAAEDGEEEGDTQMNEKNPVVPNDEEEGV>[2x]MPLCTLRQMLGEARKHKYGVGAFNVNNMEQIQGIMKAVVQLKSPVILQCSRGALKYSDMIYLKKLC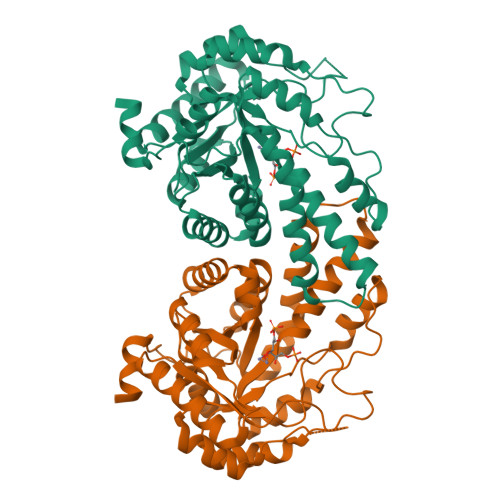EAALEKHPDIPICIHLAHGDTLESVKMAIDLGFSSVMIDASHHPFDENVRITKEVVAYAHARGVSVEAELGTLGGIEEDVQNTVQLTEPQDAKKFVELTGVDALAVAIGTSHGAYKFKSESDIRLAIDRVKTISDLTGIPLVMHGSSSVPKDVKDMINKYGGKMPDAVGVPIESIVHAIGEGVCKINVDSDSRMAMTGAIRKVFVEHPEKFDPRDYLGPGRDAITEMLIPKIKAFGSAGHAGDYKVVSLEEAKAWYK> KA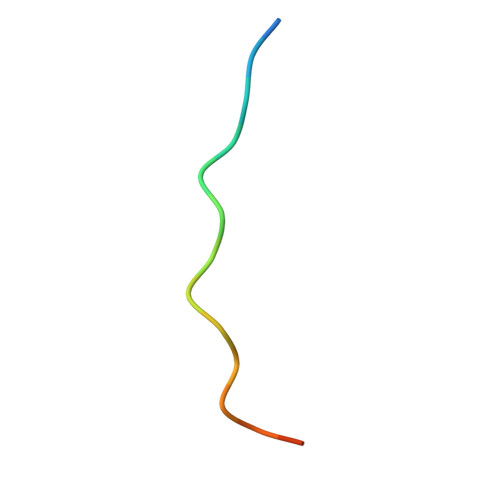FVHMPTLPNLDFHKT>[2x]MGSSHHHHHHSSGENLYFQGHMSHKVTKAHNGATLTVAVGELVEIQLPSNPTTGFAWYFEGGTKESPNESMFTVENKYFPPDSKLLGAGGTEH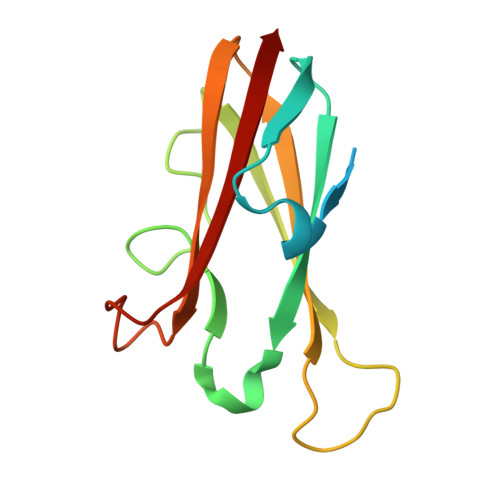FHVTVKAAGTHAVNLTYMRPWTGPSHDSERFIVYLKAN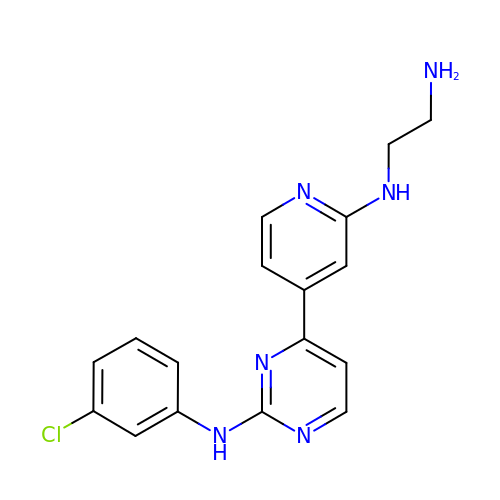N~1~-(4-{2-[(3-chlorophenyl)amino]pyrimidin-4-yl}pyridin-2-yl)ethane-1,2-diamine | C17 H17 Cl N6 | OGZKVNUWPYUXNL-UHFFFAOYSA-N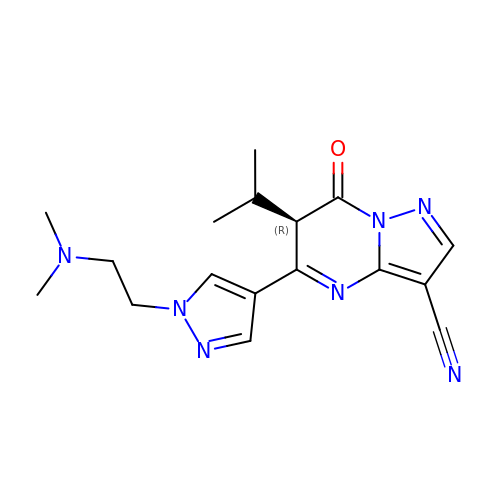5-[1-[2-(dimethylamino)ethyl]pyrazol-4-yl]-7-oxidanylidene-6-propan-2-yl-6~{H}-pyrazolo[1,5-a]pyrimidine-3-carbonitrile | C17 H21 N7 O | IHWTUDNGWXTJCT-CQSZACIVSA-N>[4x]AEAGITGTWYNQLGSTFIVT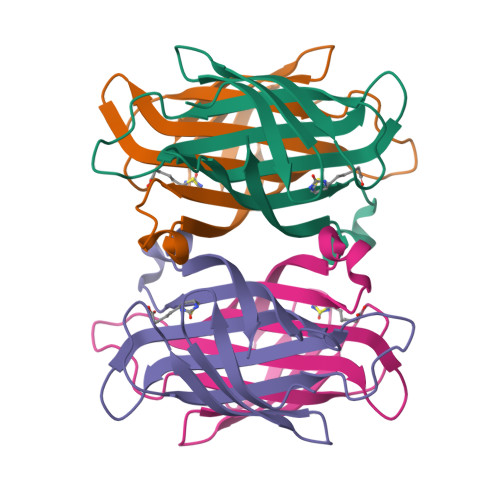AGADGALTGTFESAVGNAESRYVLTGRYDSAPATDGSGTALGWTVAWKNNYRNAHSATTWSGQYVGGAEARINTQWLLTSGTTEANAWKSTLVGHDTFTKVKPSAAS>MRGSHHHHHHGSMDKNIIIGAMTALITPFKNGKVDE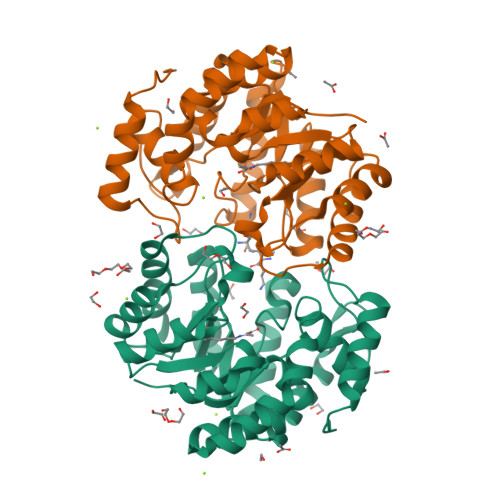QSYARLIKRQIENGIDAVVPVGTTGESATLTWEEHRTCIEIAVETCKGTKVKVLAGAGSNATHEAVGLAKFAKEHGADGILSVAPYYNKPTQQGLYEHYKAIAQSVDIPVLLYNVPGRTGCEISTDTIIKLFRDCENIYGVKEASGNIDKCVDLLAHEPRMMLISGEDAINYPILSNGGKGVISVTSNLLPDMISALTHFALDENYKEAKKINDELYNINKILFCESNPIPIKTAMYLAGLIESLEFRLPLCSPSKENFAKIEEVMKKYKIKGF[6x]>GAMDPQDEPPALDSLALDLTLRCGELRLTLAELRRLDAGTILEVTGISPGHATLCHGEQVVAEGELVDVEGRLGLQITRLVTR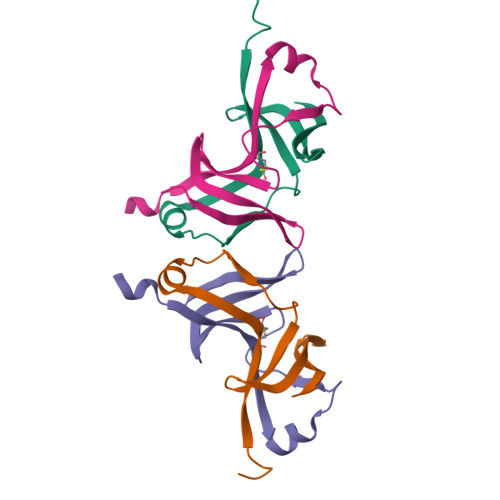S[4x]> MSRRRHSDENDGGQPHKRRKTSDANETEDHLESLICKVGEKSACSLESNLEGLAGVLEADLPNYKSKILRLLCTVARLLPEKLTIYTTLVGLLNARNYNFGGEFVEAMIRQLKESLKANNYNEAVYLVRFLSDLVNCHVIAAPSMVAMFENFVSVTQEEDVPQVRRDWYVYAFLSSLPWVGKELYEKKDAEMDRIFANTESYLKRRQKTHVPMLQVWTADKPHPQEEYLDCLWAQIQKLKKDRWQERHILRPYLAFDSILCEALQHNLPPFTPPPHTEDSVYPMPRVIFRMFDYTDDPEGPVMPGSHSVERFVIEENLHCIIKSHWKERKTCAAQLVSYPGKNKIPLNYHIVEVIFAELFQLPAPPHIDVMYTTLLIELCKLQPGSLPQVLAQATEMLYMRLDTMNTTCVDRFINWFSHHLSNFQFRWSWEDWSDCLSQDPESPKPKFVREVLEKCMRLSYHQRILDIVPPTFSALCPANPTCIYKYGDESSNSLPGHSVALCLAVAFKSKATNDEIFSILKDVPNPNQDDDDDEGFSFNPLKIEVFVQTLLHLAAKSFSHSFSALAKFHEVFKTLAESDEGKLHVLRVMFEVWRNHPQMIAVLVDKMIRTQIVDCAAVANWIFSSELSRDFTRLFVWEILHSTIRKMNKHVLKIQKELEEAKEKLARQHKRRSDDDDRSSDRKDGVLEEQIERLQEKVESAQSEQKNLFLVIFQRFIMILTEHLVRCETDGTSVLTPWYKNCIERLQQIFLQHHQIIQQYMVTLENLLFTAELDPHILAVFQQFCALQA;> MSGGLLKALRSDSYVELSQYRDQHFRGDNEEQEKLLKKSCTLYVGNLSFYTTEEQIYELFSKSGDIKKIIMGLDKMKKTACGFCFVEYYSRADAENAMRYINGTRLDDRIIRTDWDAGFKEGRQYGRGRSGGQVRDEYRQDYDAGRGGYGKLAQNQ

The nuclear cap binding complex (CBC) binds to the m7G cap of RNAs transcribed by RNA pol II. It is comprised of NCBP1 (also known as CBP80) and NCBP2 (also known as CBP20). As such, the CBC regulates gene expression at multiple levels, ranging from transcription and splicing to nuclear export and translation. The CBC promotes nuclear mRNA export through its interaction with a key mRNA export factor ALYREF.

We collected cryo-EM data from the mixture of the CBC complex and mALYREF2 in the presence of the cap analog m7GpppG. The data yielded two maps that correspond to the CBC complex and the CBC-mALYREF2 complex, respectively. The CBC map was refined to an overall resolution of 3.38 Å. The electron density of the cap analog is clearly visible bound to NCBP2. Compared to unliganded CBC, the cap analog induces significant rearrangements in both the N-terminal extension and the C-terminal tail of NCBP2 to form critical interactions. For example, the N-terminal extension (residues 16–28) swings toward the central globular domain of NCBP2 and positions the Y20 residue to sandwich the cap analog with Y43 of NCBP2. These conformational changes were also observed in the crystal structures of ligand-bound CBC. Overall, the cryo-EM structure of the CBC determined here resembles the previously reported crystal structures of the liganded CBC, with root mean squared deviation (RMSD) of 0.81 Å and 0.71 Å for NCBP1 and NCBP2, respectively.>SNARKIKTEPKQMHEDYCFQCGDGGELVMCDKKDCPKAYHLLCLNLTQPPYGKWECPWHQCDECSSAAVSFCEFCPHSFCKDHEKGAL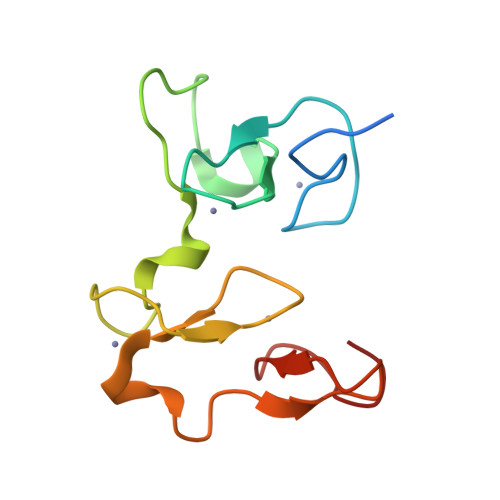VPSALEGRLCCSEHDPMAP[2x]>[2x]MVSLTERRKAETRMEIARAAARLFVGQGLRATRAEDIARAAGVAPRTFYRYFATKEEAVAPLYALGAERWVRAVREAPAELSPPEALERAVRHTLTP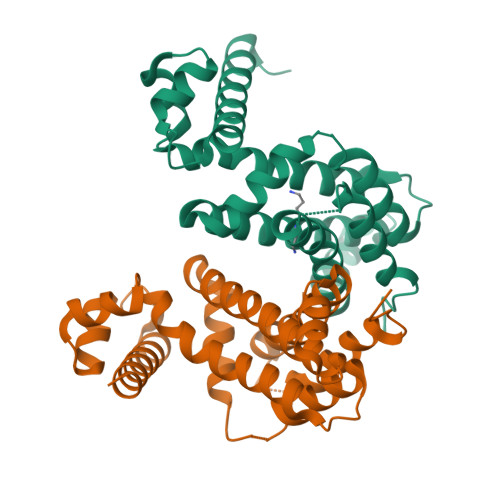GAGVSAPSWEWARTLIRLAESSPALRKVWAEVCHSTERGLVQALAARMSGGDDNVAVRLAASPRLHFAAAVAGASVRVAAEHWASSSPQGARSPLEQALLNLEVLRGFAWEAGPAEEG>MGSSHHHHHHSSRNLYFQGHMVTILILTDNVHAHALAVDLQARHGDMDVYQSPIGQLPGVPRCDVAERVAEIVERYDLVLSFHCKQRFPAALIDGVRCVNVHPGFNPYNRGWFPQVFSIIDGQKVGVTIHEIDDQLDHGPIIAQRECAIESWDSSGSVYARL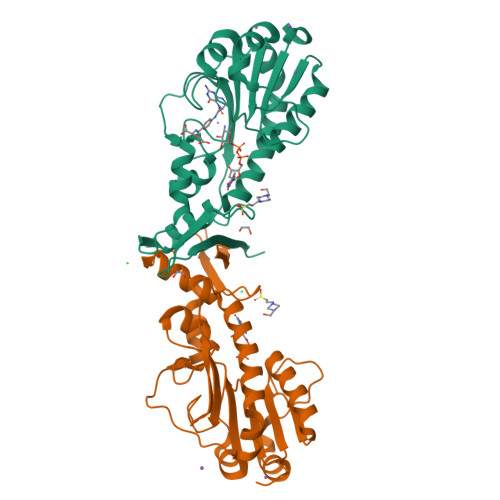MDIERELVLEHFDAIRDGSYTAKSPATEGNLNLKKDFEQLRRLDLNERGTFGHFLNRLRALTHDDFRNAWFVDASGRKVFVRVVLEPEKPAEA[2x]> GPLGSPEFPGRLEMEPDFFCVKWIPWKGEQTPIITQSTNGPCPLLAIMNILFLQWKVKLPPQKEVITSDELMAHLGNCLLSIKPQEKSEGLQLNFQQNVDDAMTVLPKLATGLDVNVRFTGVSDFEYTPECSVFDLLGIPLYHGWLVDPQSPEAVRAVGKLSYNQLVERIITCKHSSDTNLVTEGLIAEQFLETTAAQLTYHGLCELTAAAKEGELSVFFRNNHFSTMTKHKSHLYLLVTDQGFLQEEQVVWESLHNVDGDSCFCDSDFHLSHSLGKGPGAEGGSGSPE

MINDY1 and MINDY2 are members of the MINDY family of deubiquitinases (DUBs) that have exquisite specificity for cleaving K48-polyUb, yet we have a poor understanding of their catalytic mechanism. Here, we analyze the crystal structures of MINDY1 and MINDY2 alone and in complex with monoUb, di-, and penta-K48-polyUb, identifying 5 distinct Ub binding sites in the catalytic domain that explain how these DUBs sense both Ub chain length and linkage type to cleave K48-polyUb chains. The activity of MINDY1/2 is inhibited by the Cys-loop, and we find that substrate interaction relieves autoinhibition to activate these DUBs. We also find that MINDY1/2 use a non-canonical catalytic triad composed of Cys-His-Thr.

In the autoinhibited state of MINDY1, sulfur-centered hydrogen bonding of the catalytic C137 with the hydroxyl of Y114 rotates C137 away from the active site. In the active conformation, this inhibitory Y114-C137 interaction is broken due to the Cys loop movement, and the side chain of Y114 now hydrogen bonds with S163. Interestingly, in the MINDY1∼Ub complex, which represents the product-bound intermediate state, Y114 is hydrogen bonded to S163 before the transition back from the activated to the inhibited state after Ub chain hydrolysis. These observations strongly imply a linchpin role for Y114 in regulating the transition from an inhibited to active state. Disruption of this single hydrogen bond with a Y114F mutation results in increased DUB activity, with an ∼30-fold increase in kcat compared to WT. (H) A close-up image of active site of apo MINDY1 Y114F mutant compared to WT. Hydrogen bonding of C137 to Y114 is broken in the mutant. In MINDY1 and MINDY2, an additional layer of regulation is imparted by a sulfur-centered hydrogen bond between a Tyr and the catalytic Cys, which further reinforces autoinhibition.>[4x]VTPLHVQHPLDPLTKEEFLAVQTIVQNKYPISNNRLAFHYIGLDDPEKDHVLRYETHPTLVSIPRKIFVVAIINSQTHEILINLRIRSIVSDNIHNGYGFPILSVDEQSLAIKLPLKYPPFIDSVKKRGLNLSEIVCSSFTMGWFGEEKNVRTVRLDCFMKESTVNIYVRPITGITIVADLDLMKIVEYHDRDIEAVPTAENTEYQVSKQSPPFGPKQHSLTSHQPQGPGFQINGHSVSWANWKFHIGFDVRAGIVISLASIYDLEKHKSRRVLYKGYISELFVPYQDPTEEFYFKTFFDSGEFGFGLSTVSLIPNRDCPPHAQFIDTYVHSANGTPILLKNAICVFEQYGNIMWRHTENGIPNESIEESRTEVNLIVRTIVTVGNYDNVIDWEFKASGSIKPSIALSGILEIKGTNIKHKDEIKEDLHGKLVSA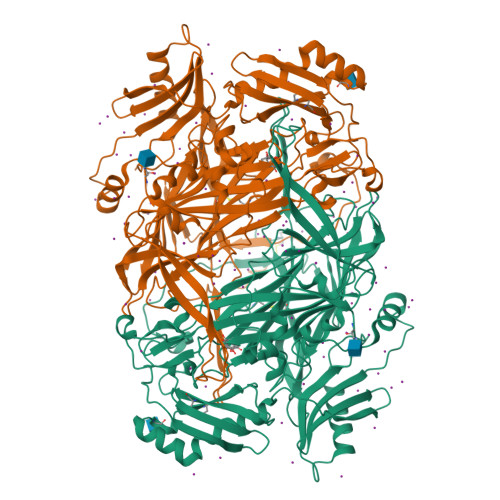NSIGIYHDHFYIYYLDFDIDGTHNSFEKTSLKTVRIKDGSSKRKSYWTTETQTAKTESDAKITIGLAPAELVVVNPNIKTAVGNEVGYRLIPAIPAHPLLTEDDYPQIRGAFTNYNVWVTAYNRTEKWAGGLYVDHSRGDDTLAVWTKQNREIVNKDIVMWHVVGIHHVPAQEDFPIMPLLSTSFELRPTNFFERNPVLKTLSPRDVAWPGCSN> SNMWVIGKSKAQDAKAIMVNGPQFGWYAPAYTYGIGLHGAGYDVTGNTPFAYPGLVFGHNGVISWGSTAGFGDDVDIFAERLSAEKPGYYLHNGKWVKMLSREE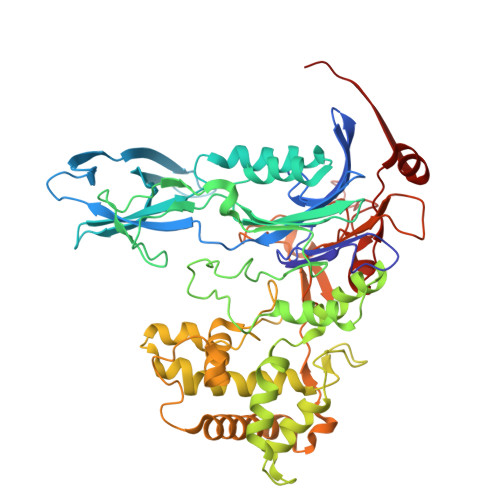TITVKNGQAETFTVWRTVHGNILQTDQTTQTAYAKSRAWDGKEVASLLAWTHQMKAKNWQEWTQQAAKQALTINWYYADVNGNIGYVHTGAYPDRQSGHDPRLPVPGTGKWDWKGLLPFEMNPKVYNPQSGYIANWANSPQKDYPASDLFAFLWGGADRVTEIDRLLEQKPRLTADQAWDVIRQTSRQDLNLRLFLPTLQAATSGLTQSDPRRQLVETLTRWDGINLLNDDGKTWQQPGSAILNVWLTSMLKRTVVAAVPMPFDKWYSASGYETTQDGPTGSLNISVGAKILYEAVQGDKSPIPQAVDLFAGKPQQEVVLAALEDTWETLSKRYGNNVSNWKTPAMALTFRANNFFGVPQAAAEETRHQAEYQNRGTENDMIVFSPTTSDRPVLAWDVVAPGQSGFIAPDGTVDKHYEDQLKMYENFGRKSLWLTKQDVEAHKESQEVLHVQR> MHHHHHHENLYFQGSGDESHYPEFSWDTVPIAFHFGKSQGLLTKEEAEFVATRSNFICLEKGHATRTHGTTEAGIEAEARQLKNLNPKMKVIFYWNTFLDYSMFAAHKEYAKHPQWWLRTTTGELDRKKGQLMRYDLSNAEFRNWWTNVAAKAVVDGTCDGVFMDAFPQIASQANRKLWGDEKFEAIQQGLQDIIQETRQKIGDDKLIVYNGIRSTPDWSAGFDFAEYTDAAMIEHFGHFQSASKETMLRDI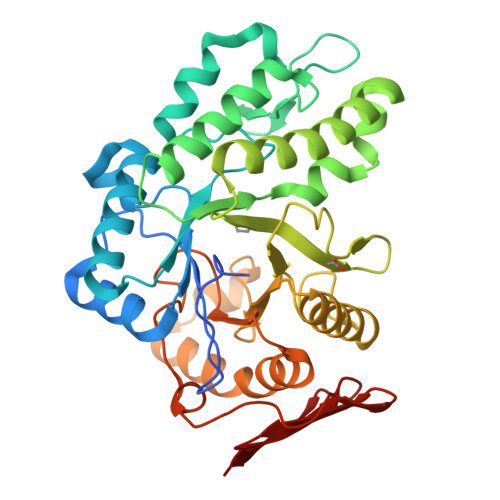LEMQRAAKAGKIVVLKGWAGFTFIDDQAMRKPLTQKRRVAKDSLKFPLACFLAGAQENCYFIYNWGYRMENGCLEWYPEFDKPLGKPVGEMVRDGWKLSREYKHASVRVDLESKEAEIRWR> SQSRIFYLRNFNNWMKSVLIGEFLEKVRQKKKRDITVLDLGCGKGGDLLKWKKGRINKLVCTDIADVSVKQCQQRYEDMKNRRDSEYIFSAEFITADSSKELLIDKFRDPQMCFDICSCQFVCHYSFESYEQADMMLRNA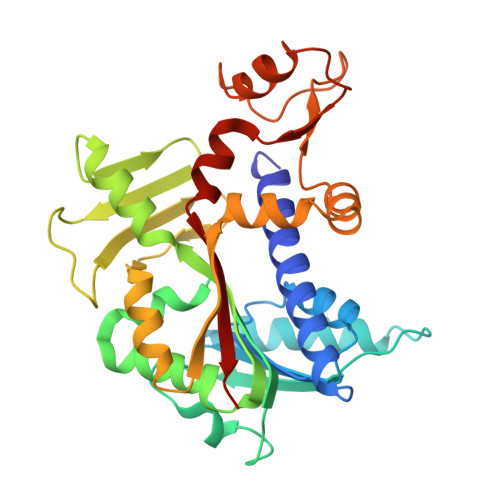CERLSPGGYFIGTTPNSFELIRRLEASETESFGNEIYTVKFQKKGDYPLFGCKYDFNLEGVVDVPEFLVYFPLLNEMAKKYNMKLVYKKTFLEFYEEKIKNNENKMLLKRMQALEPYPANESSKLVSEKVDDYEHAAKYMKNSQVRLPLGTLSKSEWEATSIYLVFAFEKQQ> APVRSLNCTLRDSQQKSLVMSGPYELKALHLQGQDMEQQVVFSMSFVQGEESNDKIPVALGLKEKNLYLSCVLKDDKPTLQLESVDPKNYPKKKMEKRFVFNKIEINNKLEFESAQFPNWYISTSQAENMPVFLGGTKGGQDITDFTMQFVSS;> LEADKCKEREEKIILVSSANEIDVRPCPLNPNEHKGTITWYK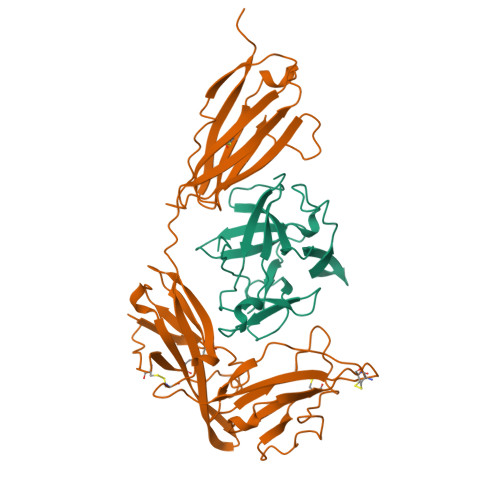DDSKTPVSTEQASRIHQHKEKLWFVPAKVEDSGHYYCVVRNSSYCLRIKISAKFVENEPNLCYNAQAIFKQKLPVAGDGGLVCPYMEFFKNENNELPKLQWYKDCKPLLLDNIHFSGVKDRLIVMNVAEKHRGNYTCHASYTYLGKQYPITRVIEFITLEENKPTRPVIVSPANETMEVDLGSQIQLICNVTGQLSDIAYWKWNGSVIDEDDPVLGEDYYSVENPANKRRSTLITVLNISEIESRFYKHPFTCFAKNTHGIDAAYIQLIYPVT> MTTVDGTANGNGAVPSTDYANGFNQNNGTSNVIDGNYMEQEEEWERAGLLDPAWEKQQRKTFTVWCNSHLRKADTQIENIEEDFRNGLKLMLLLEVISGETLPKPDRGKMRFHKIANVNKALDFIASKDVKLVSIGAEEIVDGNAKMTLGLIWTIILRFAIQDIEVEASTAKEGLLLWCQRKTSPYKNVNVHNFHNSWKDGLAFCALIHRHRPELIDYNSLTREDPVRNLNLAFDVAEKHLNIPKMLDAEDIKTSLKPD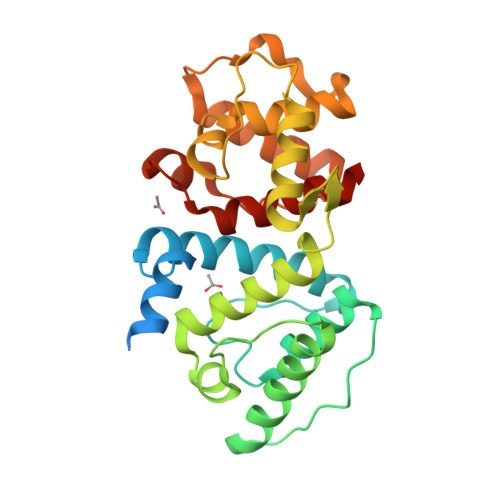ERAIMTYISSYYHTFANAQQA Phospholipases D (PLDs, EC 3.1.4.4) belong to the phospholipase superfamily and they are ubiquitously distributed in various organisms including mammals, plants and microorganisms. PLDs catalyze two kinds of reactions: (1) hydrolysis reaction, in which PLDs cleave the terminal phosphodiester bonds of phospholipids to produce phospholipid acids (PA) and the free alcohol moieties, and (2) transphosphatidylation reaction, in which PLDs transfer phosphatidic acids to acceptor alcohol moieties to form new phospholipids. In the aspect of protein structure, members in the PLD superfamily contain one or two highly conserved HxKxxxxDxxxxxxGG/S (HKD) motifs, which were assumed to act as active centers. The catalytic mechanism of PLD enzymes was well characterized to proceed through a phosphohistidine intermediate that was formed after nucleophilic attack of the phospho-substrate by the first His residue of the HKD motif (H116 in SpPLD).

In the present study, the crystal structure of a PLD from the plant-associated bacteria Serratia plymuthica strain AS9 was solved at 1.79 Angstrom (Å) resolution. Crystal structure of the ligand-free SpPLD was obtained at 1.79 Å resolution by the single-wavelength anomalous diffraction (SAD) method. Two molecules were found in one asymmetric unit, and the root-mean square deviation (RMSD) value of 307 backbone Cα between the two molecules was 0.126 Å. The overall structure of SpPLD displayed a β-α-β-α-β- sandwich fold. The structure was composed of two tightly interacting HKD domains with slightly different topology. The two HKD domains self-dimerized in close proximity to form a single active site with the catalytic histidine (H116, H311) and lysine residues (K118, K313). Two highly conserved motifs (HxKxxxxD) comprising the the putative catalytic residues His116 and His311 were found in SpPLD. The two catalytic histidine residues of the HKD motifs in SpPLD were both located at the interface of the two core β-sheets at the distance of 6.7 Å. While superimpostion and comparision the structure of SpPLD with other PLDs within the same family, an extended loop between β9 and α9 was found distinct with other PLDs. Moreover, electrostatic surface potential of SpPLD at this part showed net charge of +1, thus this loop was found positively charged.

>MHHHHHHRFDIPGYELVYTAPVETALQADDLRNTAEVWQQMFDAAKTRIDLGQFYVANQQGSLLDGVLQHLKAAGERGVKIRFLMEEKGIRLSTPETLEQLKAIPNLELRIIPYRRLSGGILHAKYLLVDGEQAFVGSQNFDWRALEHIHETGLRISDAGVVGQIQAIFEQDWRAQALLTADKPVPQLTYQPTAATPQGNYLVASPRAYNPAGVIDSQVELPRLLASAKQRVRVQVMDYAPLSYGPERSRPYYAVIDNALRSAAARGVQIELMVANWNTKKPDIAWLKSLALVPNVQIKVVTIPPASHGFIPFARVIHSKLMTIDGETAWVGTSNWTGGYLDNSRNLELVLHSPAMSQRLDTLYSQLWDSVYAEPIKLDYDYPAPKPGGES[2x]To expand the structural repertoire of determined capsid structures for the diverse Bocaparvovirus genus, viruses infecting dogs (CnMV), pigs (PBoV1), and rats (RBoV) were selected. The ORFs of these viruses coding for the major capsid protein VP2 were cloned into the pFastBac1 plasmid to enable the production of the virus-like particles (VLPs), using the Bac-to-Bac expression system in insect Sf9 cells. In the icosahedral capsid, the 60 VPs assemble via two-, three-, and fivefold symmetry-related VP interactions, resulting in pores at the fivefold symmetry axes, protrusions surrounding the threefold axes, and depressions at the twofold axes.

Canine Minute Virus (CnMV) was first isolated from German military dogs in 1967 and was initially thought to be non-pathogenic. Later, it was found to be pathogenic in newborn puppies and fetuses, as the virus was found in the lungs and intestines of nursing puppies, leading to lesions, diarrhea, and death. Following cryo-EM data collection, three-dimensional-image reconstruction of the capsids, utilizing 50,866 (CnMV), 98,388 (PBoV1), and 9199 (RBoV) individual capsid images, resulted in a resolution of 2.72, 2.31, and 2.52 Å, respectively. The high resolution of the cryo-EM maps allowed the building of reliable atomic models, starting from amino acids 34, 41, and 42 (VP2 numbering) at the N-terminus for CnMV, PBoV1, and RBoV, respectively. Capsid structures previously determined for the Bocaparvovirus genus showed disperse protrusions surrounding the threefold axis that do not significantly extend radially from the capsid surface. In contrast, the CnMV capsid shows very prominent threefold protrusions, while PBoV1 and RBoV follow the previously described characteristics of the genus. The more prominent threefold protrusions of CnMV are the result of significant insertions into VR-IV (+1 aa vs. BPV, +2 aa vs. PBoV1 and HBoV1, +4 aa vs. RBoV) and VR-VIII (+12 aa vs. PBoV1, +13 aa vs. RBoV, +15 aa vs. BPV, +17 aa vs. HBoV1). The lack of any twofold depression in CnMV is caused by an insertion in VR-III (+2 aa vs. HBoV1, +3 aa vs. PBoV1, + 6 aa vs. RBoV and BPV) and its loop conformation advancing towards the twofold symmetry axis. In contrast to VR-III, CnMV’s VR-I is the shortest loop in comparison to the other bocaviruses (−3 aa vs. BPV, −4 aa vs. HBoV1, −6 aa vs. PBoV1 and RBoV) and is located between the threefold protrusion and the fivefold region. Another feature previously observed for the bocaviruses, with the exception of GBoV1, was the presence of density extending into the interior of the capsid below the fivefold channel. This density was also seen for CnMV, but is absent in the PBoV1 and RBoV capsids.

>MEPQETENTIEADAGIAGRAGGGGGPGGGGSGGGSGVGVSTGGWEGGTLFGDNRVITVNTRQWYAPIYNGHRYTKLEGTGNTFWKGIKTPWGYFNFNAYDSHFSPQDWQRLTNEYRRWRPKKMMVKIYNLQIKQVVTLQGDTLYNNDLTAGVHIFCDGSHQYPYSQHPWDAGTMPELPYKVWLLENYGYFQFQGDLIDTSVDGGSPDVENVEKEIAKSAPFYILENANHEVLRTGEETNFHFNFDCGWVNNDRAYCPLQADFNPLVKTRRYFATRNNYNNSGKFVYTRYSPYNKPSQWMPGPSLGYIGNTQSAATREQALGPVTVVTAPPGTSAYTAFTEQQSKTNQQSASNATWSGYDVSPVNCARSGFDKIGLAYDSAPESELEEKISIRDIDNDMSRWGQVFVQDGTNKEISNDNTGQGGNTRQNMAELKNVWMFPNQAWDSTPISRDFPIWVKSPNTDKHTLFDSSDGTLPMSHPPGTIFVKVAKIPIPTQTNTDSYLTLYVTGQVTCTIEWEVERFMTKNWRPESKNDVSSFRDAFLYTVGADGTYNTPERFLEGMPTRRGINKTL[60x]> MSTYEGRWKTVKVEIEDGIAFVILNRPEKRNAMSPTLNREMIDVLETLEQDPAAGVLVLTGAGEAWTAGMDLKEYFREVDAGPEILQEKIRREASQWQWKLLRMYAKPTIAMVNGWCFGGGFSPLVACDLAICADEATFGLSEINWGIPPGNLVSKAMADTVGHRQSLYYIMTGKTFGGQKAAEMGLVNESVPLAQLREVTIELARNLLEKNPVVLRAAKHGFKRCRELTWEQNEDYLYAKLDQSRLLDTEGGREQGMKQFLDDKSI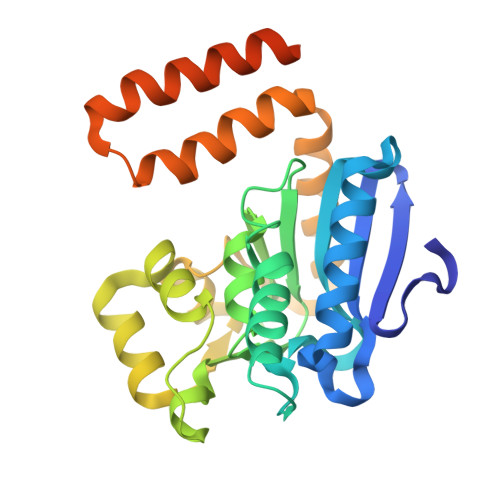KPGLQAYKR> LQHHHHHHHHASQNDTEPIVLEGKCLVVCDSNPATDSKGSSSSPLGISVRAANS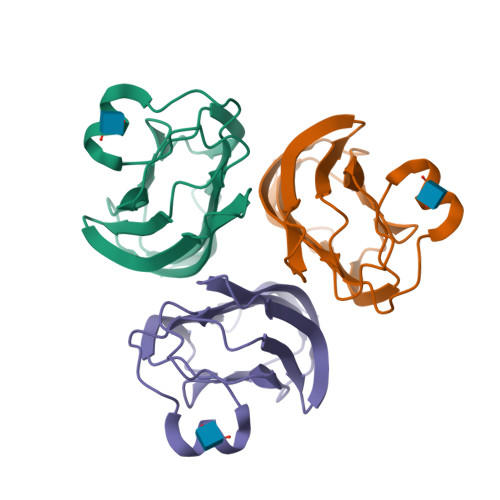KVAFSAVRSTNHEPSEMSNKTRIIYFDQILVNVGNFFTLESVFVAPRKGIYSFSFHVIKVYQSQTIQVNLMLNGKPVISAFAGDKDVTREAATNGVLLYLDKEDKVYLKLEKGNLLGGWQYSTFSGFLVFPL> SPSSSEGGAF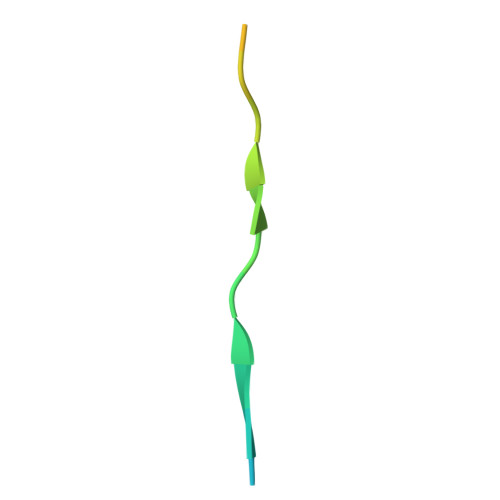TVNMPKTSTVDDIR> SIL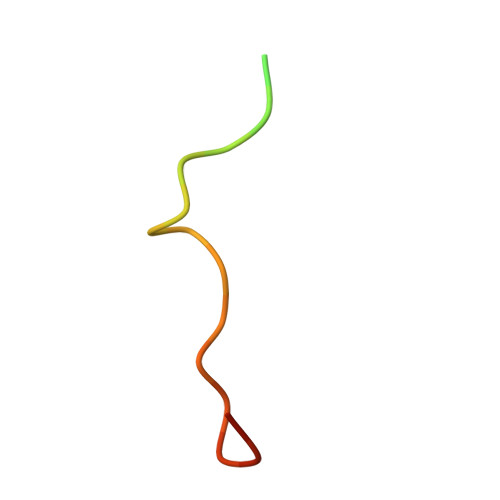YAGPTFTHSPAASNLPIPTFLHS>NLDAAGFLQIWQHFDADDNGYIEGKELDDFFRHMLKKLQPKDKITDERVQQIKKSFMSAYDATFDGRLQIEELANMILPQEENFLLIFRREAPLDNSVEFMKIWRKYDADSSGYISAAELK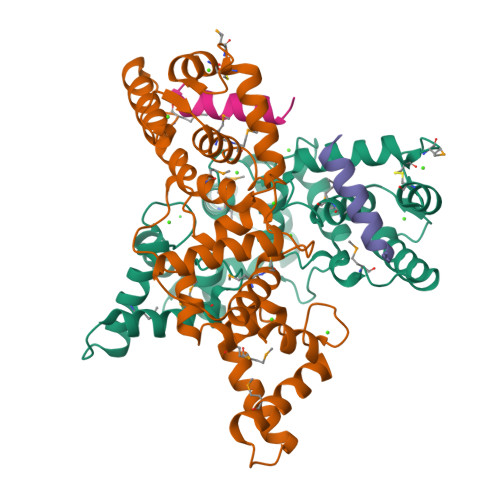NFLKDLFLQHKKKIPPNKLDEYTDAMMKIFDKNKDGRLDLNDLARILALQENFLLQFKMDASSQVERKRDFEKIFAHYDVSRTGALEGPEVDGFVKDMMELVRPSISGGDLDKFRECLLTHCDMNKDGKIQKSELALCLG[2x];>SGIIGNLRHMALDMGNE[2x]> ADVAAGSNAESYAVLCTLVQLTKATKPSVPKSKIIDEVYNVAAAIGLAIRGDAVVKNCIDKKDSKYSDLTDSDIAKKAYTERTWPVAQAGAAKLASSGEKEKYASWTHRKYTEKQKLKVHVLTAAISDVKQRADKLNKPDKLAELTGALSNSLYGNGKSNADTATLPAGGSHISMCGPADGTQGGSIVGKALKFDLICLCGKQSADSGTGEKACHEFSPLPATAIAENAAI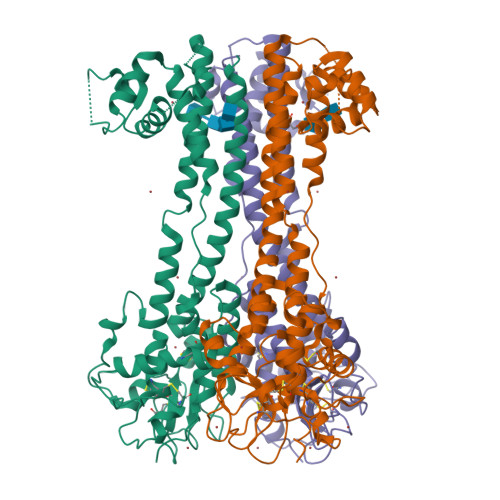NADWATIEQGCKTVAGAPSLTPESIHAALQAFYRHAGVPKGNTRNRYTTVGAPAGSGATGCDGIGGSNGGKCAAYNKAQFEAGTGPYWATQMKAAAETLVELRGQEQKLAALEAEALALNSTLDGMQHD{2-[2-(2-amino-6-oxo-1,6-dihydro-9H-purin-9-yl)ethoxy]ethyl}phosphonic acid | C9 H14 N5 O5 P | 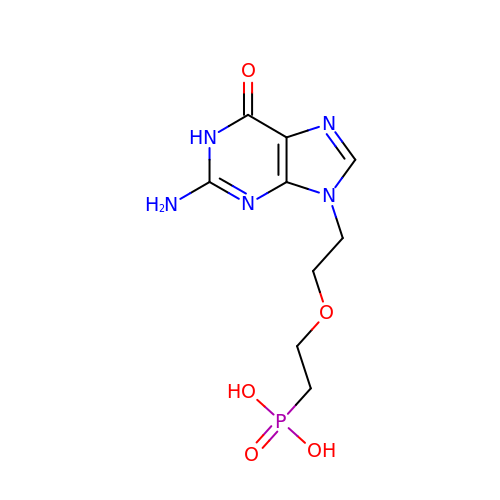KDWYBFCNTYIRFX-UHFFFAOYSA-N BACTERIORUBERIN | 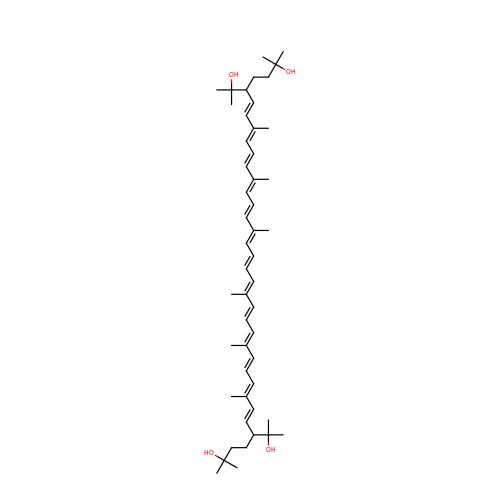C50 H76 O4 | UVCQMCCIAHQDAF-CUMPQFAQSA-N1,1-diphenylethanol | C14 H14 O 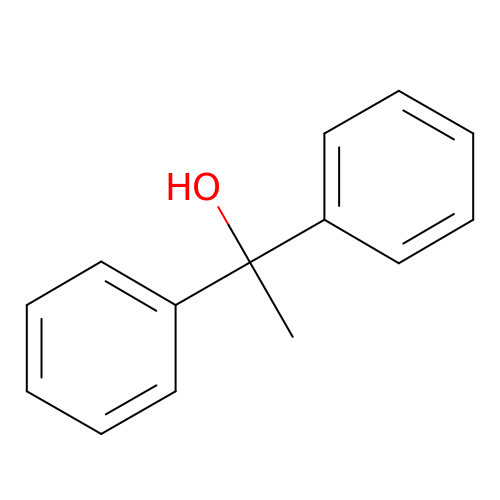| GIMDPFBLSKQRNP-UHFFFAOYSA-N>MYHHYHAFQGRKLTDQERARVLEFQDSIHYSPRYSDDNYEYRHVMLPKAMLKVIPSDYFNSEVGTLRI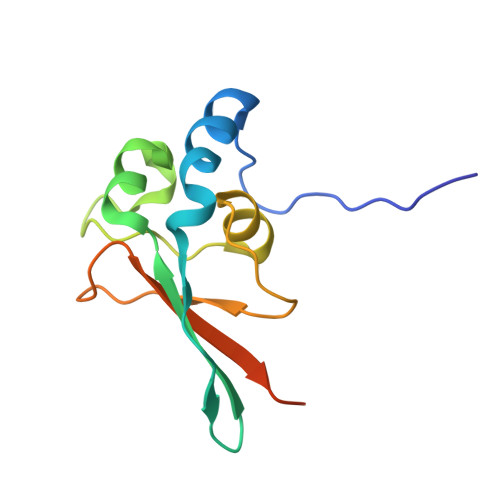LTEDEWRGLGITQSLGWEHYECHAAEPHILLFKRPLNYEAELRAATAAA[2x]>[2x]MFEQRVNSDVLTVSTVNSQDQVTQKPLRDSVKQALENYFAQ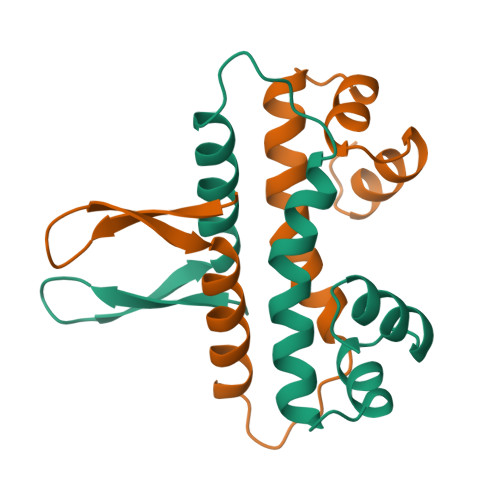LNGQDVNDLYELVLAEVEQPLLDMVMQYTRGNQTRAALMMGINRGTLRKKLKKYGMN>HMAVELNHTIVLVKDKDASATFMADLLGLPKPKEMGPFAVLQLANDVSILFMDFRGEGDIVPGHCAFLISDEEFDQIFGRIREGGIEHWADQYHREPGRINDRDGGRGVFFEDPSGHNM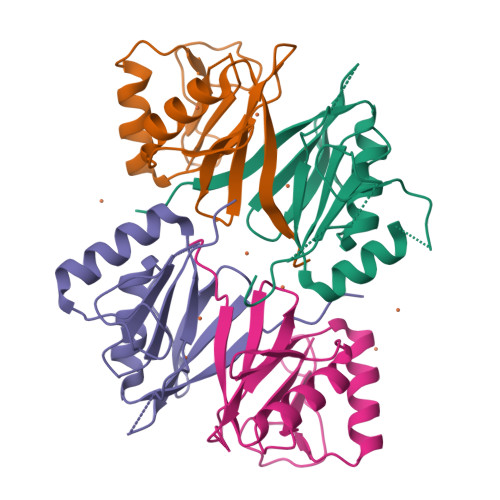EIMTRPYGSGGA[4x]> MRGSHHHHHHGIHMNSLIKENMRMMVVMEGSVNGYQFKCTGEGDGNPYMGTQTMRIKVVEGGPLPFAFDI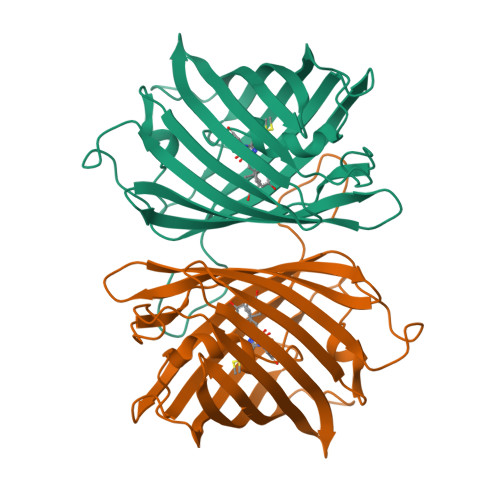LATSFMYGSKTFIKHTKGIPDFFKQSFPEGFTWERVTRYEDGGVFTVMQDTSLEDGCLVYHAKVRGVNFPSNGAVMQKKTKGWEPSTEMLYPADGGLRGYSQMALNVDGGGYLSCSFETTYRSKKTVENFKMPGFHFVDHRLERLEESDKEMFVVQHEHAVAKFCDLPSKLGRL>MAGHPLALDEAAQDLLFREARTANTFAPTHIGDEHIEAIYDLVKWGPTSMNQQPMRVVLVRSDESRRALLQHVLEGNRDKVASAPLVAVLAADLSFPDTLPRLFPHAPNARHAYADENARRESAVFNTALQLGYFIIGIRAGGLAAGPIAGFDPEGVHKEFFPGEPVLVTSIVNIGYPGPDAFSARLPRLGYREVVR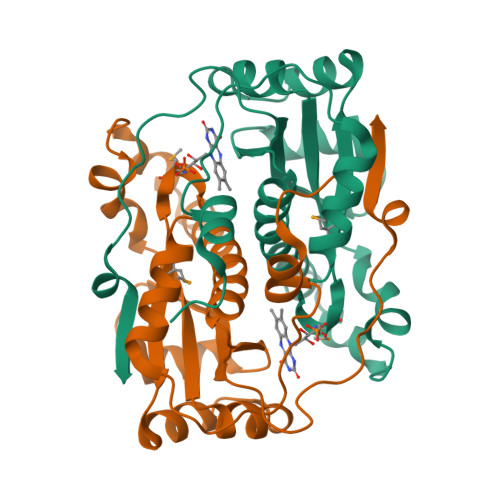SV[2x]> MSWFDPNWNPFFNRSIIVSGNLVVAGGVIEGNGGGLTNSAFSNPDTIRTDLTGNVTSNGTVRSSLIQTNSIVASGDAYANVWNGNAAFITGISANTTLVGNVRISISGNLTGNFAVSTTTVSNTMTANVLIGTTLTVNNLSATRANVQVLTGNVTGNVRLIANVVNVAAYTVGNLTTSSNVSTTNLNVTSNINGNVRSSTANVQGRLSATTPTTGSIISSSFIANSFTSSGNVQIGDFFGNVRASVGTFDMIASNVFSNVANIIEIRSDIISNIANVGNGTFVFVNASNITTTNITGNITSNVASFSNVDSIFGNVGNLRANTLTVTYANITGTLASGNVAVGNLISADNTSEFANITSFTTNGLVVNGNIIAAIGNGNVFLANVITANSLTLQSSSSTAASNVTTTRWIQSTTSTSNVMTIGNITSGNVISSNAAYFANVISNTITVMSAMTVSGNVSFGNVSFGNVSYGNITANVTTSTGNVSVDNLTSNVVN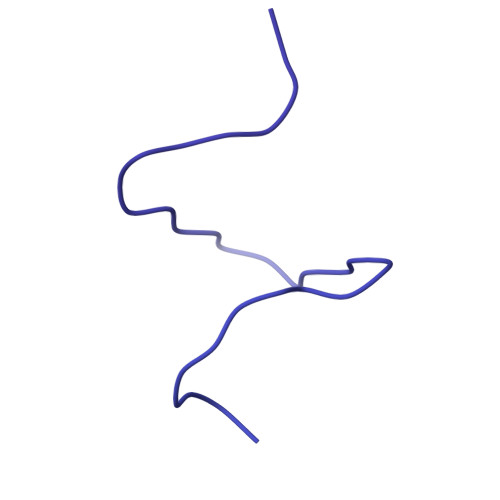VVFCNASSVTANTLTSIALTGNTYVYSANTGVLTANVGNVFGTLTVGVANVTSMVSNALFANTAVVSNLSVSNLTVTISSDISNISITGNTSGNVFAANIATIGTLNTANVVANLVASNVMNAWVTSNIRTLITGNANVSTTTSNVITTGGFTITGNITSGLLTSNVIAGNITMYNTSNTTLFTSNTSNIANFFAGNMTAVNTIVSNLEIQGNSVVITQTTPFKVTSVLLANVLFANTIISNTFTTTANVVGNISTDIANIGIANVNFLNTTDFAVNTANIVNYTPTSNINVTGNLTLGNANIVNFYATSANIVGNITANNAVITFLTTPFYKGSGTVSAGFTSIISANALSNVIVFGNLSANIVVSNTLLSNSINVATVFSNVVNIGQVTSTGTTLVNSINFNISNVDVSGNVLVTRDVYTTNISVTTANIANVTFFSNVAIGNLISTRNLTAANLISSSDLFNSGPYTSSQNVTIDTLNFTAGNLGTVAARTTITTPTLFATDVNFTQDALVAGELITQNFYGNITSANIGSRITIGNANVTQTNITGNVVIPRTSNAAGFNSRLLISNNTTVTSNIVANSLISTGNIITNLLQTTGQVSFASLAVEYIDVANLAVRNVVTIGGNLTVSNVANLFSITANTVNMSTVTTNTLSANTITGTSNVLVAGNIIGNCFGNVLVNRGVVTGNVFADTITVPLNAVGVLTGNALIVPNTALHSVAITGSSAFTSNIRTLNTPNAFIWNTSVPSSGLLDARRLRFSQYITSNRIVEMRYFYITNALPQKYDSGGLNARYDLSFGTTLPTSQGQTWHHFLNTLYIGAQYNTNFSINCLIINATTTGLEVIIYNPFGIAASLSSSTPELYFYITSIATSTQ> MGQSEKQEEPDYPINKFMNTTDEIWVFRTTQENVQKCKKDKNKYMTTSATFFTRSHEEQDQIHEQELVGKFANFYDKPDGVYDRIDITGDKTGVYEEALAYASKENTCGVVGVWAFDGETTVVWRELRVRNRPNDATKVDEMCKKKFDDY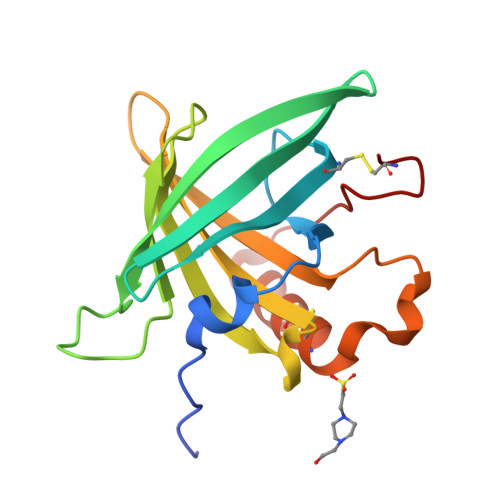VQVVNKSWTSPYNEKCK> GGGDFTTCLETESINWNCTGPFLNLGNCQKQQKKEPYTNIATQLKGLKAISVLDVPIITGIPDDIAGALRYIEEKEDFHVQLTIEYAMLSKYCDYYTQFSDNSGYSQTTWRVYLRSHDFEACILYPNQHFCRCVKNGEKCSSSNWDFANEMKDYYSGKQTKFDKDLNLALTALHHAFRGTSSA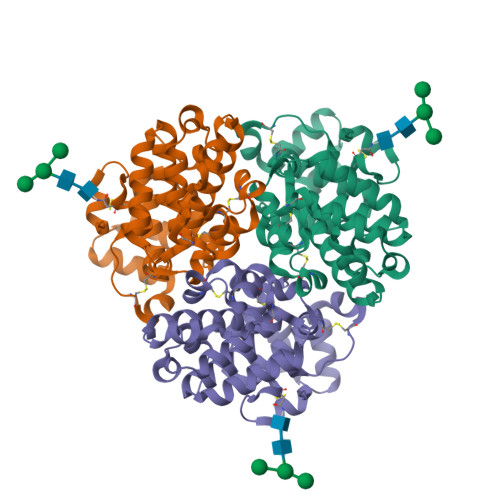YIATMLSKKSNDDLIAYTNKIKTKFPGNALLKAIIDYIAYMKSLPGMANFKYDEFWDELLYKPNPAK>[2x]MSSDADAHKVGLIPVTLMVSGNIMGSGVFLLPANLASTGGIAIYGWLVTIIGALGLSMVYAKMSFLDPSPGGSYAYARRCFGPFLGYQTNVLYWLACWIGAIAMVVIGVGYLSYFFPILKDPLVLTITCVVVLWIFVLLNIVGPKMITRVQAVATVLALIPIVGIAVFGWFWFRGETYMAAWNVSGLG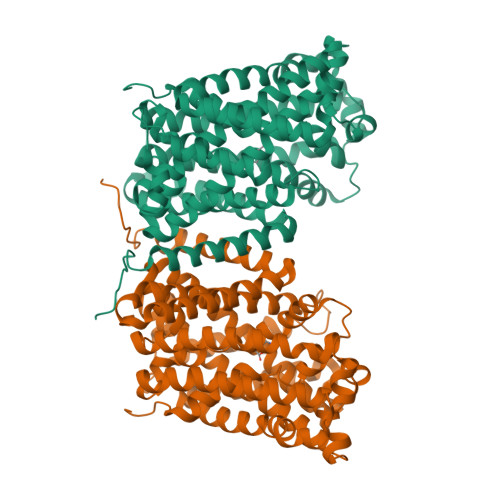TFGAIQSTLNVTLWSFIGVESASVAAGVVKNPKRNVPIATIGGVLIAAVCYVLSTTAIMGMIPNAALRVSASPFGDAARMALGDTAGAIVSFCAAAGCLGSLGGWTLLAGQTAKAAADDGLFPPIFARVNKAGTPVAGLIIVGILMTIFQLSSISPNATKEFGLVSSVSVIFTLVPYLYTCAALLLLGHGHFGKARPAYLAVTTIAFLYCIWAVVGSGAKEVMWSFVTLMVITAMYALNYNRLHKNPYPLDAPISKD> AIPQKIRIG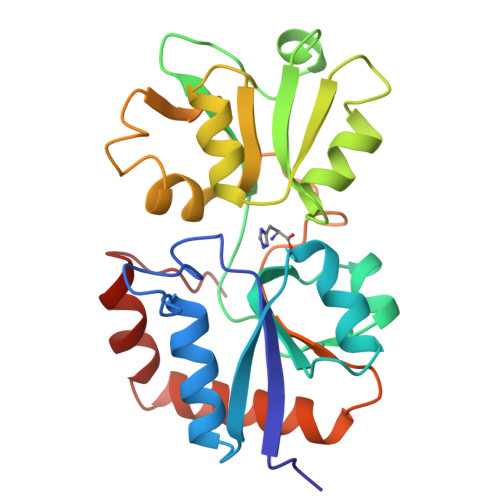TDPTYAPFESKNAQGELVGFDIDLAKELCKRINTQCTFVENPLDALIPSLKAKKIDAIMSSLSITEKRQQEIAFTDKLYAADSRLVVAKNSDIQPTVASLKGKRVGVLQGTTQETFGNEHWAPKGIEIVSYQGQDNIYSDLTAGRIDAAFQDEVAASEGFLKQPVGKDYKFGGPAVKDEKLFGVGTGMGLRKEDNELREALNKAFAEMRADGTYEKLAKKYFDFDVYGG> GHMPYKVSTPPAVDSSEVPAAGEPPLPLVVPPTPVGGNALGGCGIITAPGSAPAPGDVSAEAWLVADLDSGAVIAARDPHGRHRPASVIKVLVAMASINTLTLNKSVAGTADDAAVEGTKVGVNTGGTYTVNQLLHGLLMHSG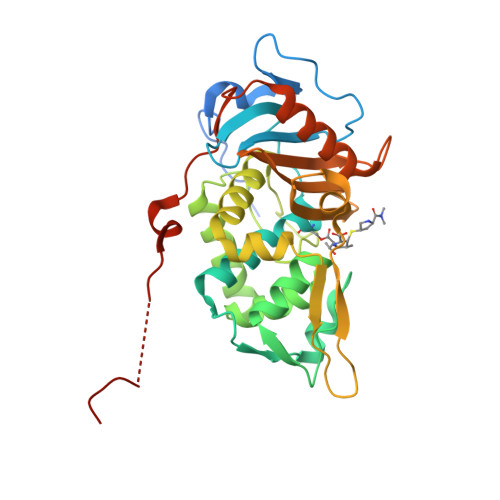NDAAYALARQLGGMPAALEKINLLAAKLGGRDTRVATPSGLDGPGMSTSAYDIGLFYRYAWQNPVFADIVATRTFDFPGHGDHPGYELENDNQLLYNYPGALGGKTGYTDDAGQTFVGAANRDGRRLMTVLLHGTRQPIPPWEQAAHLLDYGFNTPAGTQIGTLIEPDPSLMSTDRNPADRQRVDPQAAAR> GQRGWFCGSVSQDLRQFWVAEGGTISDPRAADFLFSCDASHPDTLRIYQSLDYIEDNATVFHAYYLSAVANAKIKNSVALGHFILPPACLQKEIRRKIGSFIWEQDQ;> YRCSGCIAVEKSLNSRNFSKLLHSCPYQCDRHKVIVEAEDRYKSELRKSLICNKKILLTP

TERB1 is a molecular scaffold that simultaneously interacts with TERB2 and shelterin subunit TRF1. Knockout of any components of the TERB1–TERB2–MAJIN (TTM) complex impairs the telomere–NE attachment and results in infertility in both male and female mice. In the present study, we characterize the TERB1–TERB2 and TERB2–MAJIN interactions and determine the crystal structures of the N-terminal domains of TERB2 and MAJIN in complex with TERB2-binding motif of TERB1 and MAJIN-binding motif of TERB2, respectively. To reveal the structural basis for the interactions between TERB1 and TERB2 and between TERB2 and MAJIN, we crystallized the TERB1587–659–TERB22–116 and the TERB2119–220–MAJIN2–149 complexes and determined their structures using single-wavelength anomalous dispersion (SAD) method at resolutions of 3.3 and 2.9 Å, respectively.

To gain further insight into the telomere recruitment function of the TTM complex, we first characterized the interaction between TERB1 and TERB2 using bimolecular fluorescence complementation (BiFC) assay. We found that a short fragment of TERB1 consisting of residues 587–636, which is adjacent to the TRF1-binding motif (TERB1TBM, residues 642–656) of TERB1, was necessary and sufficient for binding with the N-terminal domain of TERB2 (residues 1–116). The TERB1T2BM–TERB2NTD complex adopts a compact globular fold, resembling a single folding unit. TERB2NTD consists of a three-stranded β sheet (β1–β2–β3) at one end and six α helices that flank the β sheet and scatter at the periphery of the structure. TERB1T2BM is a helix–turn–helix (HtH) motif with a long tail that folds back to the middle turn between the two helices. Notably, Cys592 and Cys595 at the N-terminus of the tail together with Cys618 and His621 in the middle of the HtH motif chelate a Zn2+ ion, playing a key role in defining the overall shape of TERB1T2BM. TERB1T2BM adopts an extended conformation and packs against the concaved surface of TERB2NTD, burying ~1400 Å2 of surface area at the interface. The long helix H2 of TERB1T2BM fits into a large hydrophobic groove formed by helices α3 and α6 and loops L33 and L56 of TERB2NTD through extensive contacts involving a panel of hydrophobic residues at both sides of the interface. Helix H1 and the N-terminal tail of TERB1T2BM pack against a flat hydrophobic surface of TERB2NTD formed by the β sheet and helices α3 and α5. Most notably, a cluster of acidic and polar residues in TERB2NTD (Asp55, Glu58, Asp59, and Gln110) mediate a network of salt bridge and hydrogen-bonding interactions with positively charged residues in helices H1 and H2 of TERB1T2BM (Arg605, Arg629, Lys632, and Arg636), helping secure the HtH motif of TERB1T2BM on the surface of TERB2NTD.> GPLGSPEFMALAVAPWGRQWEEARALGRAVRMLQRLEEQCVDPRLSVSPPSLRDLLPRTAQLLREVAHSRRAAGGGGPGGPGGSGDFLLIYLANLEAKSRQVAALLPPRGRRSANDELFRAGSRLRRQLAKLAIIFSHMHAELHALFPGGKYCGHMYQLTKAPAHTFWRESCGARCVLPWAEFESLLGTCHPVEPGCTALALRTTIDLTCSGHVSIFEFDVFTRLFQPWPTLLKNWQLLAVNHPGYMAFLTYDEVQERLQACRDKPGSYIFRLSCTRLGQWAIGYVSSDGSILQTIPANKPLSQV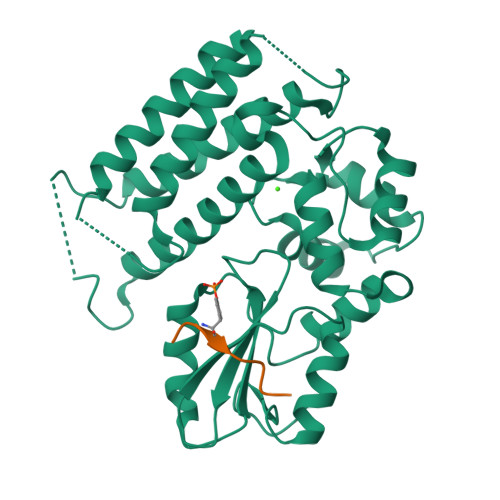LLEGQKDGFYLYPDGKTHNPDLTELG;> EDSFLQRYSSDPT>GDAYAQWLADGGPSSGRPP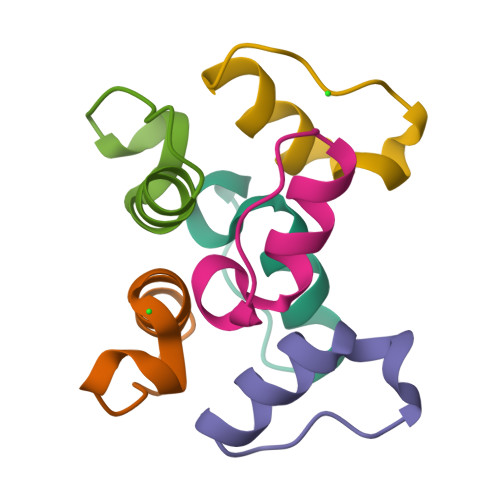PSG[6x]> MTEQLQMTRRTMLAGAALAGAVAPLLHTAQAHAAGAAAAAGAAPVDISTLPRVKVDLVKPPFVHAHDQVAKTGPRVVEFTMTIEEKKLVIDREGTEIHAMTFNGSVPGPLMVVHENDYVELRLINPDTNTLLHNIDFHAATGALGGGALTQVNPGEETTLRFKATKPGVFVYHCAPEGMVPWHVTSGMNGAIMVLPRDGLKDEKGQPLTYDKIYYVGEQDFYVPKDEAGNYKKYETPGEAYEDAVKAMRTLT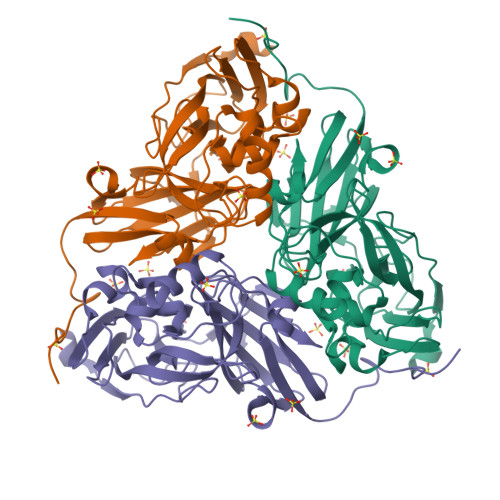PTHIVFNGAVGALTGDHALTAAVGERVLVVHSQANRDTRPHLIGGHGDYVWATGKFRNPPDLDQETWLIPGGTAGAAFYTFRQPGVYAYVNHNLIEAFELGAAGHFKVTGEWNDDLMTSVVKPASM> GGGUUAUGUGUGCCCGGCAUGGGUGCAGUCUAUAGGGUGAG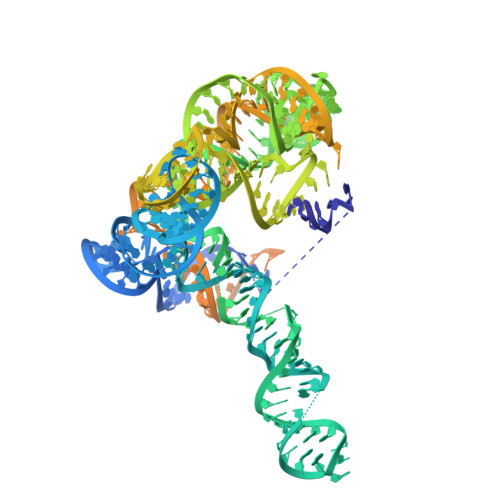AGUCCCGAACUGUGAAGGCAGAAGUAACAGUUAGCCUAACGCAAGGGUGUCCGUGGCGACAUGGAAUCUGAAGGAAGCGGACGGCAAACCUUCGGUCUGAGGAACACGAACUUCAUAUGAGGCUAGGUAUCAAUGGAUGAGUUUGCAUAACAAAACAAAGUCCUUUCUGCCAAAGUUGGUACAGAGUAAAUGAAGCAGAUUGAUGAAGGGAAAGACUGCAUUCUUACCCGGGGAGGUCUGGAAACAGAAGUCAGCAGAAGUCAUAGUACCCUGUUCGCAGGGGAAGGACGGAA>MSLSVELRDATVDDLSGIMEIYNDAVVNTTAIWNEVVVDLENRKDWFAARTSRGFPVIVAILDGKVAGYASYGDWRAFDGYRHTREHSVYVHKDARGHGIGKRLMQALIDHAGGNDVHVLIAAIEAENTASIRLHESLGFRVVGRFS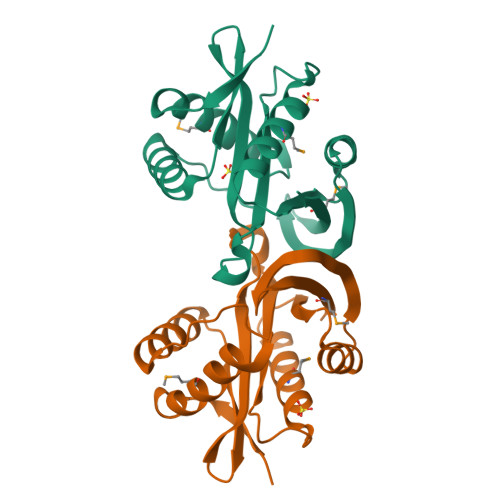EVGTKFGRWLDLTCMELKLGEGHHHHHH[4x]Native amine dehydrogenases (nat‐AmDHs) have recently emerged as a potentially valuable new reservoir of enzymes for the sustainable and selective synthesis of chiral amines, catalyzing the NAD(P)H‐dependent ammoniation of carbonyl compounds with high activity and selectivity. MATOUAmDH2, recently identified from the Marine Atlas of Tara Oceans Unigenes (MATOUv1) database of eukaryotic genes, displays exceptional catalytic performance against its best identified substrate, isobutyraldehyde, as well as having broader substrate scope than other nat‐AmDHs. In the interests of providing a platform for the rational engineering of this and other nat‐AmDHs, we have determined the structure of MATOUAmDH2 in complex with NADP+ and also with the cofactor and cyclohexylamine. The two‐domain structure of the MATOU monomer is similar to that observed with CfusAmDH and MsmeAmDH, with a largely N‐terminal Rossman fold domain (residues 8–158; 309–351) and a largely C‐terminal domain 159–309 comprising a seven‐stranded beta sheet.

The first structure of the amine dehydrogenase MATOUAmDH2 was determined in complex with NADP+ to a resolution of 2.32 Å. The crystals were obtained in space group P212121 and featured four molecules in the asymmetric unit, comprising two dimers and permitting observation of open and closed conformers of the enzyme subunits. Electron density for the backbone and side chains could be modelled for most regions save for residues 189–193 and 190–193 in monomers C and D respectively. The cofactor NADP+ was bound within the cleft between the two domains in each monomer. The monomers that constitute each dimer (A/D and B/C) in the asymmetric unit presented two distinct conformations: a more open form (subunits B and D), and a much more closed form (A and C), where loops had closed over the active site containing the NADP+. The closed monomers show that the major contributions to this closure are the loops in the beta sheet domain, most especially those between residues P240 and G255 and Y171 and E190. The loop closure serves to form the active site and to bring many amino acid residues within closer proximity to bound ligands. A superimposition of the open and closed forms shows that Y176 and L180 have moved into position as a result of the loop movement and consequent active site closure. Open and closed forms of AmDH monomers were also observed in a single structure of the amine dehydrogenase AmDH4 from Petrotoga mobilis (6G1 M) although that enzyme is different from MATOUAmDH2 in binding and transforming keto acid substrates. Monomers within the structure are representative of more open and closed conformations of the enzyme and illustrate the profound changes undergone by nat‐AmDHs during the catalytic cycle.

>MHHHHHHSPLRVALYGFGNQNKEMAKMLVERKDVEIVAVISNKSNVGKDFGEVIGLAPQGILVTAGLDAAETLRTTNPQIAMLSTLSTVGDIESQLRACAENKVNVYTIAEELTFSWTSAPEKTKEMDELFKEHNVSLIGGGFLDGACCDMARTMAAMMHKIDKLDGGLQYNVDHYGQVLAIAHGVGLSEEEFYAENGPGWTSPTSYPKSYVYNMNDWFASAFGLTVIKTEEVKTPTKAPIELYSEAIGRAIPVGQCTGMIVTATTTTEEGVIIVEKQVGKCYEDGDEDMVFMNLEGNPTGGVGFTMKNPPTPAMTNTIAISRMFQTVDAPAGYITTDKLPTMEAYVHGRL[4x]3-{6-[(2-CHLOROPHENYL)AMINO]-1H-INDAZOL-3-YL}-5-{[4-(DIMETHYLAMINO)BUTANOYL]AMINO}BENZOIC ACID | C26 H26 Cl N5 O3 | 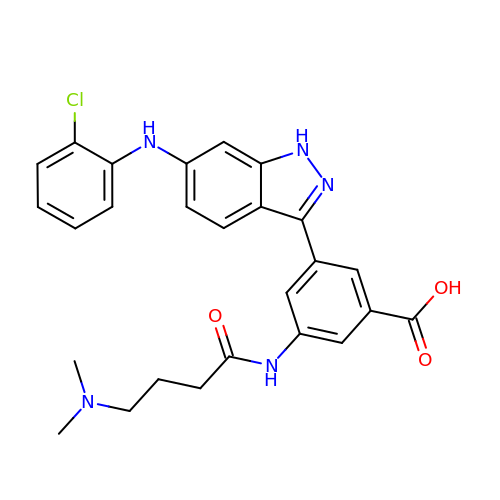QHYSKDAWIUFROA-UHFFFAOYSA-N> MEEVITIAQIVHRGTDILSLNNEEIEALVDEIYSTLKGSNDIKNIRLIDFLFTLKDFVNHVRAEQSKLPDLSMPIEAYIRQLLVDPDVVPIVSEKKKELRVRPSTRKEIFLINGTHLAVPAEAPIEIYGLKLRLKTFSPQCFMRMAEIGSFSPETLGYVASGANLTNFIRVFMKCVDQETWKKNGEGVVVTTKENIIQFTHQYIELYKFLRSGGHSWLINRLAEEMVHRKLDREDQGSHISNIVETEEIEPEENIKRVIFFLKELSTMYSVSPVFTSGYMPLLYDLYRAGYLEVLWNPVEQKFLQHAEQREKEQMILQQVDMKLTEVITQARQYFKIMEEKIGRVQSDAIREILTMEGKVDDPNSILQEVIKACGKQEAELITTEYLNIKKQWELQEKNACAHLKLVKQLRSGLQYAELLKVLESIRVLYKEKNNTTNWNLCKACGFKLLCPHVDMLIQLQAAEASYDTMRTKLMKFSGINKEKENNQGLIYSYFCKICGEELAHFIQEDRTADVGIIGDLNSKLRVFIWQETMKACTFIHFGKLVDVKQFANIAVNVCLPLVYSIENIKKEEDYDPLTQLYAVIYIYAYILNLIYSSQKNKEFLTITIHGMKADSSLNAYVTFLLEKMMQQYSGIINQLSEITDQWIANNFREAFKKIIHQNGLQGLSVQDDTKVLLTEILLDPMYDYAATVARIDGSIPMHKPRTPKEAEYEFKTVIGRTPAELLSQKEFYDKIYTSKYRPDFTQLTRLNDIYFQEESLRVWWGGRDEEKTSTLIYLRAYELFLKYLQNAPNFNSELAEFKTYENAYGEQKALLAQQGFYNIFDPNTGRADQRTRLFEYKRLPISTLYDERGLPHKWTIYVYKAVDSSQKPAEIEVTRKDVIKKIDNHYALADLRCSVCHVLQHEVGQLNIKKVQTALKASLEFNTFYAFYESRCPKGGLHDFQDKKCVKCGLFTYIIYDHLSQPELVHDYYNNYKDQYDKEKMSIRSIQIKKDMTTPSTETQPKPPQEPWTFDYGKIIKTAKILDISPAVIEAIGAMEGRSYADIREGQGAPPPPTSMDD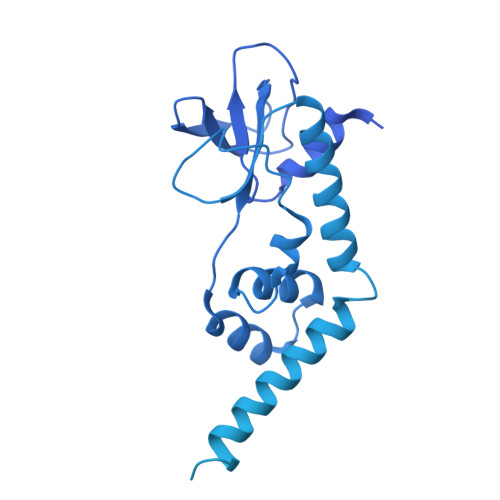PRLMAVDSAVRIFLYNYNCLRHVSTFNKPPIHVERLVKHLSYEEKEDLEKVLPNVVNEYHTTFKHLRVTDPASALLYSIEFLCISFLTLYEIKEPSWVVNIVREFALTELNTIIQSEKLLSKPGAFNFMIFGEDFVCSGEDSSMDDISAYSSPGLFGEDIIDRLDDPFSIEDVDISLDVLDNLAPQ> MASWSHPQFEKGAENLYFQSNAMKLAQGAFVDVIRIGALSPPTDQRSLWARTLLSEAVDQGLDSLPVPLQDVSTFTVTLQPALAVRLKALADQHNTPVSVYAAGLIEAMRRRSESGSVAEAPMELPADALPGEGAVREVLRPLLKQAAEKTAAGKIVFAEAATGTGKGRMIASLAAAAAIKGDTVVVSAPLAVTWQLVNDMKDIPEVRRVGLTLSLGRPNFISPQRTLEWAIDNERADLAAWIEGGGKPLSLRSMETSKVISHELCWLLEDALLLAEDLPADSLLLTSEDPADCPAQQLYVAMRSNYTEAGIILCSHFMLAAHTRMMQMRGLGNDEELDDEAPTGLSLPH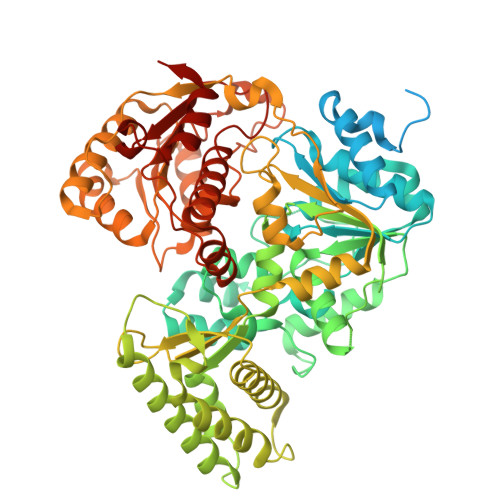FIDTLIVDEAHLLEQAFASVYTHTLRLRPLMRTIEGLGSRGRKPALDALKELFTQMQVASARSTNTSLNVPLSDVPELIPALKDTVKTLGALPTKGMSRDARSVIRIATRAANDALSGHSRLRIEVTPVHSYPMLLSGRSNLQRALLGLWNATGGATLVSATLFTTGDNGSLTRWKLEVPTERAAFLPPVHPAWTTAPVLLHKEFCAHEPDDSPEWATECAQTIQGVASTAQGGTLVLCTSYQNTELLAGRLGAALGDRLIVQSKTSSAATCLAQFKAKHKAGIRPVWLGLGAAWTGIDLSDHSLPDNPELDRLLSDLVITRIPVGQNRSLTHERRTAIGGFRIISQEAAWHFRQGLGRLVRRPGVTHKNLWVLDARIYGGAAWVAPFRQILDRYKKA>MQIRDWLPLLGMPLMLLFVQIIAIVLVMPMQAAGLVAFENPSSVANPLIFIGMLLAFTLVLLVLLRTGGRRFIAAFIGFALFMTFLYIFGALSLLALGPTTAAAAGTLIGAVAVTALLYLYPEWYVIDILGVLISAGVASIFGISLEPLPVLVLLVLLAVYDAISVYRTKHMITLAEGVLETKAPIMVVVPKRADYSFRKEGLNISEGEERGAFVMGMGDLIMPSILVVSSHVFVDAPAVLWTLSAPTLGAMVGSLVGLAVLLYFVNKGNPQAG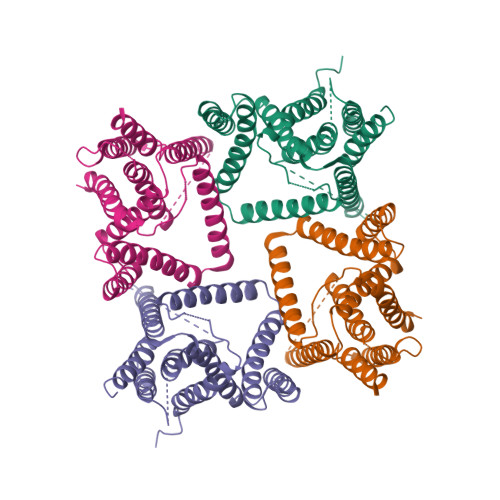LPPLNGGAILGFLVGAALAGSFSWLPF[4x]>MEAVLNELVSVEDLLKFEKKFQSEKAAGSVSKSTQFEYAWCLVRSKYNDDIRKGIVLLEELLPKGSKEEQRDYVFYLAVGNYRLKEYEKALKYVRGLLQTEPQNNQAKELERLIDKAMKKDGLLEVLFQ[2x]

A tetratricopeptide repeat (TPR) motif containing mitochondrial outer membrane protein, mitochondrial fission protein 1 (Fis1), mediates mitochondrial fission by recruiting large cytosolic GTPase, Drp1, to the mitochondrial outer membrane. The cytosolic domain of Fis1 is composed of 6 tight α-helices with two anti-parallel TPR motifs forming a concave hydrophobic surface. Fis1 interaction with Drp1 occurs during cellular stress, but not under physiological conditions, suggesting that cellular signals during stress activate Fis1. Human Fis1 protein contains a single cysteine, Cys41, in the entire protein.

To explore this possibility further, we crystallized and determined the X-ray structures of the WT and three phosphorylation mimic-mutants of Fis1: Thr34Asp Fis1, Thr34Glu Fis1 and Tyr38Glu Fis1. Consistently, we observed that the first 30 residues including the α1 helix were missing from the structure providing strong evidence that the α1 helix undergoes significant conformational change and is potentially disordered in the phosphorylated forms, whereas it was intact in the WT. Unlike phosphorylation mimic mutants, the WT Fis1 crystallized as a non-covalent dimer. We rationalized that the α1-helix and N-terminus structure are intact in WT Fis1, making Cys41 unavailable for disulfide bridge formation and hence WT Fis1 could not form a covalent dimer. We observed that the concave hydrophobic surface that is known to mediate protein-protein interactions in TPR motif-containing proteins is between the interface of the dimer in both our current and the previously reported structure. We therefore hypothesized that the WT dimer observed by X-ray crystallography was an artifact due to crystal packing and the dimer of Fis1 should be different in solution. Indeed, the dimer structure determined from crystallography did not fit the SAXS curve, suggesting that the Fis1 dimer in solution is structurally different than that observed in the crystal. When we modeled the structure of Fis1 WT dimer using the Thr34Asp Fis1 covalent dimer with modeled the missing unstructured first 30 residues, the Fis1 covalent WT dimer perfectly fitted the SAXS curve for WT Fis1 dimer. The modeled WT Fis1 covalent dimer fitted both the P1 and P2 symmetry enforced ab initio envelops independently calculated from the experimental SAXS curve. This evidence indicates that the Fis1 dimer that is present in solution is not related to the WT crystallographic dimer; these data combined with the data from the non-reducing non-heat denatured SDS-PAGE gel suggest that the small amount of Fis1 dimer in solution is indeed a covalent dimer. However, it is also possible that the differences of WT Fis1 dimers in solution and crystals may represent different types of dimers that enable interactions with different protein partners.>[2x]MKAVCVMRGEEGVKGVVHFTQAGDAVKVHAEFEGLKPGKHGFHVHEFGDT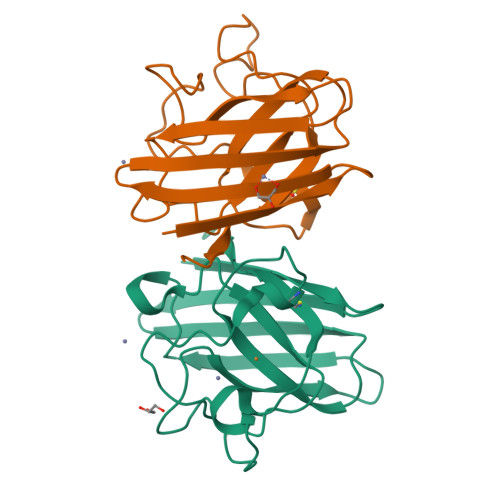TQGCTSAGAHFNPHGKNHGAPDAAERHVGDLGNVTAGADGKATLDLTDKMISLTGEHSVIGRSLVIHVDPDDLGLGGHELSLITGNAGGRVACGIIGIAKSE>[3x]MAQVQQLTPAQQAALRNQQAMAANLQARQIVLQQSYPVIQQVETQTFDPANRSVFDVTPANVGIVKGFLVKVTAAITNNHATEAVALTDFGPANLVQRVIYYDPDNQRHTETSGWHLHFVNTAKQG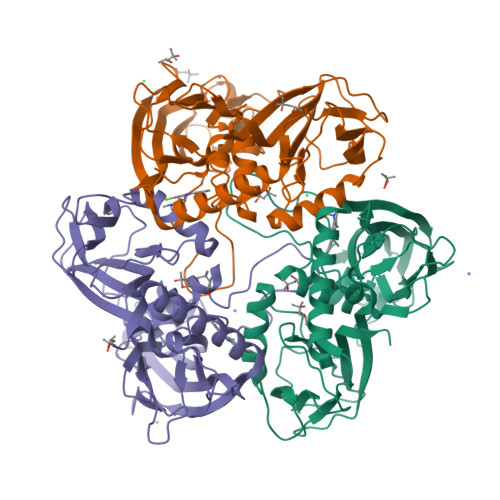APFLSSMVTDSPIKYGDVMNVIDAPATIAAGATGELTMYYWVPLAYSETDLTGAVLANVPQSKQRLKLEFANNNTAFAAVGANPLEAIYQGAGAADCEFEEISYTVYQSYLDQLPVGQNGYILPLIDLSTLYNLENSAQAGLTPNVDFVVQYANLYRYLSTIAVFDNGGSFNAGTDINYLSQRTANFSDTRKLDPKTWAAQTRRRIATDFPKGVYYCDNRDKPIYTLQYGNVGFVVNPKTVNQNARLLMGYEYFTSRTELVNAGTISTT> GSHML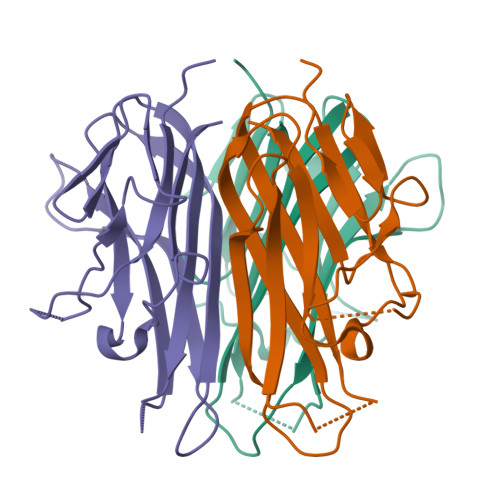KGQEFAPSHQQVYAPLRADGDKPRAHLTVVRQTPTQHFKNQFPALHWEHELGLAFTKNRMNYTNKFLLIPESGDYFIYSQVTFRGMTSESSEIRQAGRPNKPDSITVVITKVTDSYPEPTQLLMGTKSVCEVGSNWFQPIYLGAMFSLQEGDKLMVNVSDISLVDYTKEDKTFFGAFLL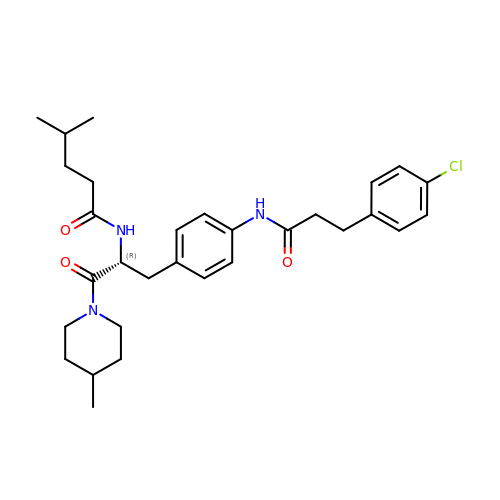N-[(2R)-3-(4-{[3-(4-chlorophenyl)propanoyl]amino}phenyl)-1-(4-methylpiperidin-1-yl)-1-oxopropan-2-yl]-4-methylpentanamide | C30 H40 Cl N3 O3 | LEQKKFVJROREDY-HHHXNRCGSA-N Naphthalene 1,2-dioxygenase from Pseudomonas putida strain NCIB 9816-4 (NDO) is one of the most well studied Rieske dioxygenases; it is an α3β3 hexamer and is the first Rieske nonheme iron oxygenase for which the three-dimensional structure was determined. The α subunit of NDO contains a Rieske [2Fe–2S] center that accepts electrons from the ferredoxin component, which originate from an NAD(P)H on a reductase component, and transfers them to a nonheme mononuclear iron at the active site. The catalytic domain of the terminal oxygenase is the well described 2-His/carboxylate center composed of a mononuclear iron coordinated by two histidines and one aspartic acid inside a large hydrophobic active site. NDO has a relaxed substrate specificity and catalyzes the dioxygenation of many two-ring and three-ring aromatic compounds to their respective cis-dihydrodiols.

In the case of 1-chloronaphthalene, NDO dihydroxylates the nonhalogenated ring. The C atoms on the same side of the molecule as the Cl atom are in the closest proximity to the modeled dioxygen. This results in the formation of (1R,2S)-8-chloro-1,2-dihydro­naphthalene-1,2-diol as the major product and (1R,2S)-5-chloro-1,2-dihydronaphthalene-1,2-diol as the minor product. The structure of NDO in complex with 1-choloronaphthalene was determined to 1.5 Å resolution. The Cl atom was found to sit near the entrance of the active site in an area that is relatively open.

> MNYNNKILVSESGLSQKHLIHGDEELFQHELKTIFARNWLFLTHDSLIPAPGDYVTAKMGIDEVIVSRQNDGSIRAFLNVCRHRGKTLVSVEAGNAKGFVCSYHGWGFGSNGELQSVPFEKDLYGESLNKKCLGLKEVARVESFHGFIYGCFDQEAPPLMDYLGDAAWYLEPMFKHSGGLELVGPPGKVVIKANWKAPAENFVGDAYHVGWTHASSLRSGESIFSSLAGNAALPPEGAGLQMTSKYGSGMGVLWDGYSGVHSADLVPELMAFGGAKQERLNKEIGDVRARIYRSHLNCTVFPNNSMLTCSGVFKVWNPIDANTTEVWTYAIVEKDMPEDLKRRLADSVQRTFGPAGFWESDDNDNMETASQNGKKYQSRDSDLLSNLGFGEDVYGDAVYPGVVGKSAIGETSYRGFYRAYQAHVSSSNWAEFEHASSTWHTELTKT;> INIQEDKLVSAHDAEEILRFFNCHDSALQQEATTLLTQEAHLLDIQAYRAWLEHCVGSEVQYQVISRELRAASERRYKLNEAMNVYNENFQQLKVRVEHQLDPQNWGNSPKLRFTRFITNVQAAMDVNDKELLHIRSNVILHRARRGNQVDVFYAAREDKWKRGEGGVRKLVQRFVDYPERILQTHNLMVFL> MASSSGAGAAAAAAAANLNAVRETMDV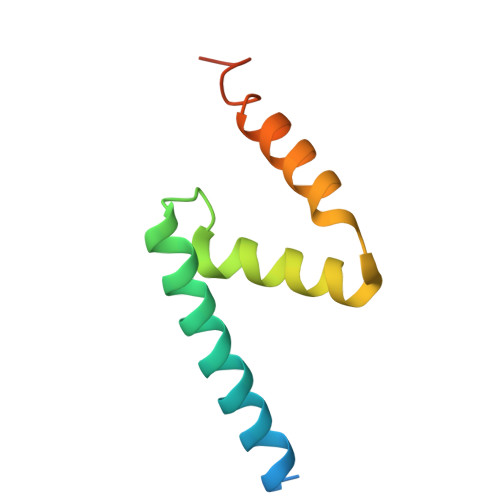LLEISRILNTGLDMETLSICVRLCEQGINPEALSSVIKELRKATEALKAAENMTS> MKPSEMRNLQATDFAKEIDARKKELMELRFQ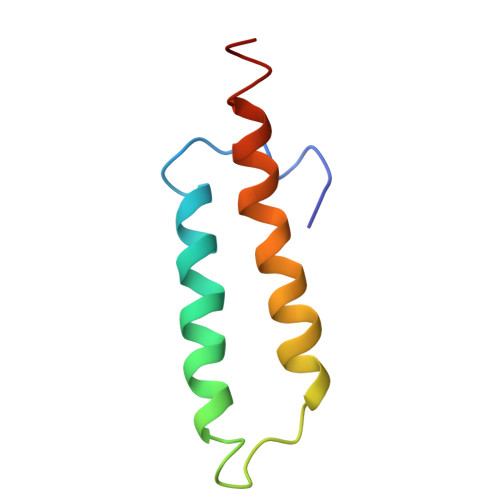AAAGQLAQPHRVRQLRREVAQLNTVKAELARKGEQQ>LPDSVDWREKGCVTEVKYQGSCGACWAFSAVG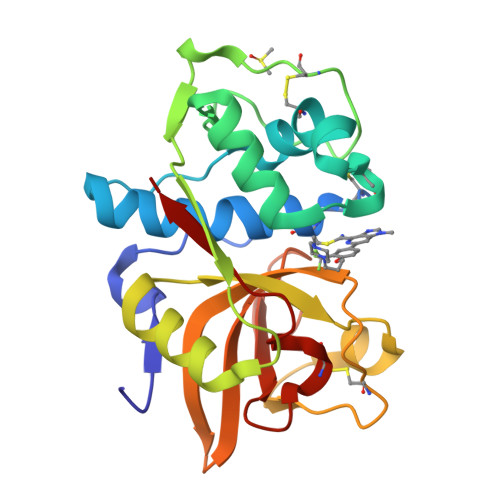ALEAQLKLKTGKLVSLSAQNLVDCSTEKYGNKGCNGGFMTTAFQYIIDNKGIDSDASYPYKAMDQKCQYDSKYRAATCSKYTELPYGREDVLKEAVANKGPVSVGVDARHPSFFLYRSGVYYEPSCTQNVNHGVLVVGYGDLNGKEYWLVKNSWGHNFGEEGYIRMARNKGNHCGIASFPSYPEI[2x]The majority of traits controlled by rhl transcription factor RhlR depend on PqsE, a dispensable thioesterase in Pseudomonas Quinolone Signal (PQS) biosynthesis that interferes with RhlR through an enigmatic mechanism likely involving direct interaction of both proteins. Here we show that PqsE and RhlR form a 2:2 protein complex that, together with RhlR agonist N-butanoyl-L-homoserine lactone (C4-HSL), solubilizes RhlR and thereby renders the otherwise insoluble transcription factor active. PqsE is a thioesterase that triggers transcription of the RhlR regulon through a hitherto cryptic mechanism, which we identify here as involving a significant chaperone-like component that enhances the stability of RhlR via protein complex formation. In common with many other gram-negative bacteria, two QS circuits use N-acyl-L-homoserine lactones (HSLs) as autoinducers, namely N-(3-oxododecanoyl)-L-HSL (3-oxo-C12-HSL) and N-butanoyl-L-HSL (C4-HSL), which are produced by autoinducer synthases LasI and RhlI and activate the LuxR-type transcription factors LasR and RhlR, respectively.

Indeed, the PROSS-designed RhlR-P75, in which 75 (out of 241) residues were mutated with respect to the original sequence, could easily be produced in E. coli, even in the absence of C4-HSL or mBTL. It crystallized readily in the presence of C4-HSL or mBTL, but not without these ligands. A complex with mBTL diffracted to 2.15 Å resolution and yielded well-resolved electron density for the ligand. A complex with C4-HSL was less well resolved (3.5 Å resolution), but the shape of the electron density confirms similar interactions. Co-expression of RhlR-P75 and His6-tagged PqsE revealed that the interaction between both proteins has been lost by the introduced mutations.

>MRNDGGFLDWWEDLRSEMQSITDSQEVFAVLEKEVRRLGFDYYAYCVRHPIPFTRPRIFMFGNYPPAWQEHYQAQNYFAIDPTIRHCLRSGNHIVWSDDLFADAQELWDDARDYGLRHGATHSCMAPNGVMGFLSVARSSPAISPHEREELRLRMRCLIELLHQTLTELNHPSLQPQPICLSKREREILRWTADGKTSAEIAKILGISESTVNFHLKNIQKKFNAPNKTQAAAYAAALGLI[4x]[[[(3~{a}~{R},4~{R},6~{R},6~{a}~{R})-4-(2-azanyl-7-methyl-6-oxidanylidene-1~{H}-purin-7-ium-9-yl)-2,2-dimethyl-3~{a},4,6,6~{a}-tetrahydrofuro[3,4-d][1,3]dioxol-6-yl]methoxy-oxidanyl-phosphoryl]oxy-sulfanyl-phosphoryl] 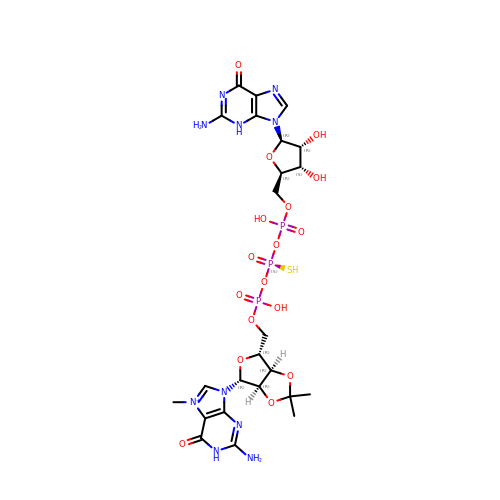[(2~{R},3~{S},4~{R},5~{R})-5-(2-azanyl-6-oxidanylidene-3~{H}-purin-9-yl)-3,4-bis(oxidanyl)oxolan-2-yl]methyl hydrogen phosphate | C24 H34 N10 O17 P3 S | DSKLYZYSTSOTOM-RGGYBXOHSA-O> MKDLLKFLKAQTKTEEFDAIKIALASPDMIRSWSFGEVKKPETINYRTFKPERDGLFCARIFGPVKDYECLCGKYKRLKHRGVICEKCGVEVTQTKVRRERMGHIELASPTAHIWFLKSLPSRIGLLLDMPLRDIERVLYFESYVVIEGGMTNLERQQILTEEQYLDALEEFGDEFDAKMGAEAIQALLKSMDLEQECEQLREELNETNSETKRKKLTKRIKLLEAFVQSGNKPEWMILTVLPVLPPDLRPLVPLDGGRFATSDLNDLYRRVINRNNRLKRLLDLAAPDIIVRNEKRMLQEAVDALLDNGRRGRAITGSNKRPLKSLADMIKGKQGRFRQNLLGKRVDYSGRSVITVGPYLRLHQCGLPKKMALELFKPFIYGKLELRGLATTIKAAKKMVEREEAVVWDILDEVIREHPVLLNRAPTLHRLGIQAFEPVLIEGKAIQLHPLVCAAYNADFDGDQMAVHVPLTLEAQLEARALMMSTNNILSPANGEPIIVPSQDVVLGLYYMTRDCVNAKGEGMVLTGPKEAERLYRSGLASLHARVKVRITEYEKDANGELVAKTSLKDTTVGRAILWMIVPKGLPYSIVNQALGKKAISKMLNTCYRILGLKPTVIFADQIMYTGFAYAARSGASVGIDDMVIPEKKHEIISEAEAEVAEIQEQFQSGLVTAGERYNKVIDIWAAANDRVSKAMMDNLQTETVINRDGQEEKQVSFNSIYMMADSGARGSAAQIRQLAGMRGLMAKPDGSIIETPITANFREGLNVLQYFISTHGARKGLADTALKTANSGYLTRRLVDVAQDLVVTEDDCGTHEGIMMTPVIEGGDVKEPLRDRVLGRVTAEDVLKPGTADILVPRNTLLHEQWCDLLEENSVDAVKVRSVVSCDTDFGVCAHCYGRDLARGHIINKGEAIGVIAAQSIGEPGTQLTMRTFHIGGAASRAAAESSIQVKNKGSIKLSNVKSVVNSSGKLVITSRNTELKLIDEFGRTKESYKVPYGAVLAKGDGEQVAGGETVANWDPHTMPVITEVSGFVRFTDMIDGQTITRQTDELTGLSSLVVLDSAERTAGGKDLRPALKIVDAQGNDV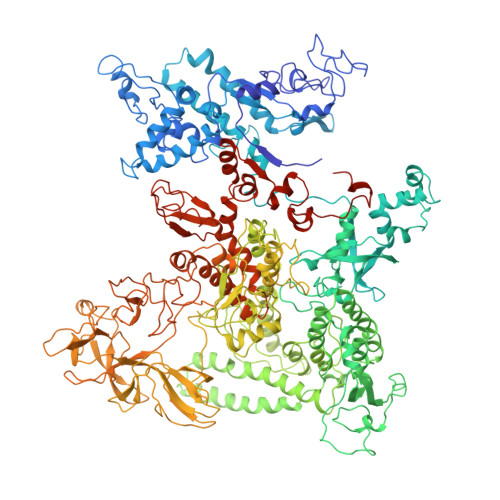LIPGTDMPAQYFLPGKAIVQLEDGVQISSGDTLARIPQESGGTKDITGGLPRVADLFEARRPKEPAILAEISGIVSFGKETKGKRRLVITPVDGSDPYEEMIPKWRQLNVFEGERVERGDVISDGPEAPHDILRLRGVHAVTRYIVNEVQDVYRLQGVKINDKHIEVIVRQMLRKATIVNAGSSDFLEGEQVEYSRVKIANRELEANGKVGATYSRDLLGITKASLATESFISAASFQETTRVLTEAAVAGKRDELRGLKENVIVGRLIPAGTGYAYHQDRMRRRAAGEAPAAPQVTAEDASASLAELLNAGLGGSDNEHHHHHH>MATRIAILGAGPSGMAQLRAFQSAQEKGAEIPELVCFEKQADWGGQWNYTWRTGLDENGEPVHSSMYRYLWSNGPKECLEFADYTFDEHFGKPIASYPPREVLWDYIKGRVEKAGVRKYIRFNTAVRHVEFNEDSQTFTVTVQDHTTDTIYSEEFDYVVCCTGHFSTPYVPEFEGFEKFGGRILHAHDFRDALEFKDKTVLLVGSSSSAEDIGSQCYKYGAKKLISCYRTAPMGYKWPENWDERPNLVRVDTENAYFADGSSEKVDAIILCTGYIHHFPFLNDDLRLVTNNRLWPLNLYKGVVWEDNPKFFYIGMQDQWYSFNMFDAQAWYARDVIMGRLPLPSKEEMKADSMAWREKELTLVTAEEMYTYQGDYIQNLIDMTDYPSFDIPATNKTFLEWKHHKKENIMTFRDHSYRSLMTGTMAPKHHTPWIDALDDSLE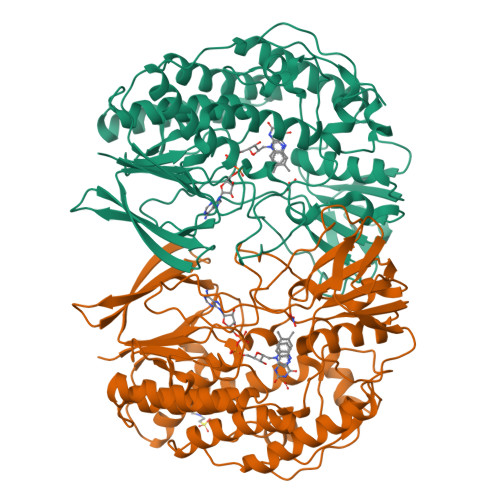AYLSDKSEIPVAKEALEHHHHHH[3x]> MVHHHHHHSSGEHTGQSAAATMPLDSIDVSIPELFYNDSVGEYFKRLRKDDPVHYCADSAFGPYWSITKYNDIMHVDTNHDIFSSDAGYGGIIIDDGIQKGGDGGLDLPNFIAMDRPRHDEQRKAVSPI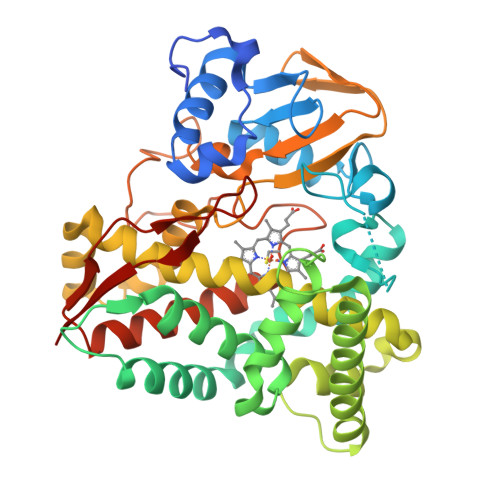VAPANLAALEGTIRERVSKTLDGLPVGEEFDWVDRVSIEITTQMLATLFDFPFEERRKLTRWSDVTTAAPGGGVVESWDQRKTELLECAAYFQVLWNERVNKDPGNDLISMLAHSPATRNMTPEEYLGNVLLLIVGGNDTTRNSMTGGVLALHKNPDQFAKLKANPALVETMVPEIIRWQTPLAHMRRTAIADSELGGKTIRKGDKVVMWYYSGNRDDEVIDRPEEFIIDRPRPRQHLSFGFGIHRCVGNRLAEMQLRILWEEILTRFSRIEVMAEPERVRSNFVRGYAKMMVRVHA>MGPLWGPLYAPVSESMSKFDTATVLSVHHWTDTLFSFTCTRDQALRFNNGEFTMVGLEVDGKPLTRAYSIVSPNYEEHLEFFSIKVQNGPLTSRLQHLKVGDPVLIGKKPTGTLVADNLLPGKTLWMLSTGTGLAPFMSIIRDPDIYERFDKV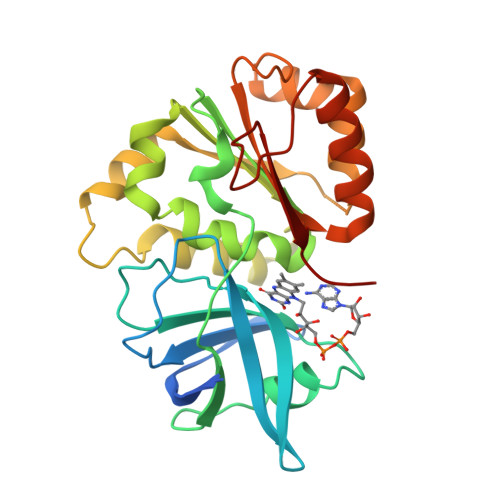VLTHTCRLKGELAYMDYIKHDLPGHEYLGDVIREKLVYYPTVTREEFENEGRITDLIASGKLFTDLDMPPFSPEQDRVMLCGSTAMLKDTTELLKKAGLVEGKNSAPGHYVIERAFVD[2x]> MVDYIVEYDYDAVHDDELTIRVGEIIRNVKKLQEEGWLEGELNGRRGMFPDNFVKEIKRETE;> PARPPKPR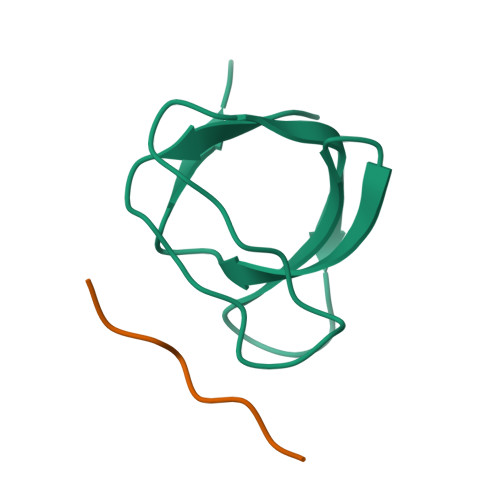PRR> MGHHHHHHAENLYFQGHMLRLSAPGQLDDDLCLLGDVQVPVFLLRLGEASWALVEGGISRDAELVWADLCRWVADPSQVHYWLITHKHYDHCGLLPYLCPRLPNVQVLASERTCQAWKSESAVRVVERLNRQLLRAEQRLPEACAWDALPVRAVADGEWLELGPRHRLQVIEAHGHSDDHVVFYDVRRRRLFCGDALGEFDEAEGVWRPLVFDDMEAYLESLERLQRLPTLLQLIPGHGGLLR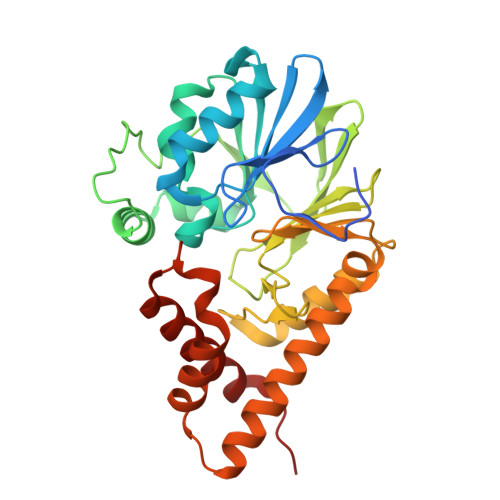GRLAADGAESAYTECLRLCRRLLWRQSMGESLDELSEELHRAWGGQSVDFLPGELHLGSMRRMLEILSRQALPLD> LGSSNDNIELVDFQNIMFYGDAEVGDNQQPFTFILDTGSANLWVPSVKCTTAGCLTKHLYDSSKSRTYEKDGTKVEMNYVSGTVSGFFSKDLVTVGNLSLPYKFIEVIDTNGFEPTYTASTFDGILGLGWKDLSIGSVDPIVVELKNQNKIENALFTFYL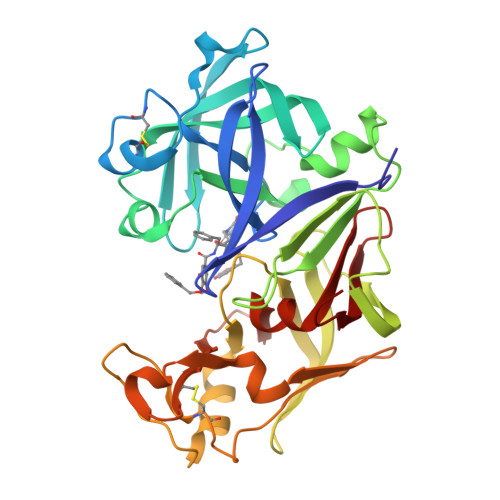PVHDKHTGFLTIGGIEERFYEGPLTYEKLNHDLYWQITLDAHVGNIMLEKANCIVDSGTSAITVPTDFLNKMLQNLDVIKVPFLPFYVTLCNNSKLPTFEFTSENGKYTLEPEYYLQHIEDVGPGLCMLNIIGLDFPVPTFILGDPFMRKYFTVFDYDNHSVGIALAKKNL> GSAMGQNPWATTTAFADFMKRFNIPQVHGSGIFVDLGRDTEGYREVGGKCPVFGKAIQMHQPAEYSNNFLDDAPTSNDASKKPLPGGFNNPQVYTSGQKFSPIDDSLLQERLGTAGPKTAIGRCALYAYSTIAVNPSTNYTSTYKYPFVYDAVSRKCYVLSVSAQLLKGEKYCSVNGTPSGLTWACFEPVKEKSSARALVYGSAFVAEGNPDAWQSACPNDAVKDALFGKWEDGQCVPFDTKTSVQSDQATNKEECWKRVFANPLVASDAPTTYPEAAQKNWNDFWPVHEQSSPKSGGFGANWANFYLEKESGETICAIFDQVPDCFAPITGAVAYTALGSSTEVNLPQCDSASFIPIEGPCNNCVQVVTECVGNQFDQTSKACCTEPEAAALVPR;> GSASDIAQFLTDSGMKAIEDCSWNPIMQQMACVVVAGSGS

AMA1, a type I transmembrane protein, is conserved across all Apicomplexans and its knockdown has been shown to markedly reduce invasion. Recently, Toxoplasma sporozoites were subjected to detailed transcriptomic and proteomic analyses. It was found that, in addition to the well-characterized “generic” AMA1 and RON2, sporozoites also express two paralogues dubbed sporoAMA1 and sporoRON2, respectively, that are not expressed at detectable levels in tachyzoites or bradyzoites. To better understand the mutually exclusive nature of the interaction between the sporozoite and generic AMA1/RON2 pairings, we set out to solve the crystal structure of apo sporoAMA1 and of sporoAMA1 bound to a portion of sporoRON2-D3 (sD3). The results presented here demonstrate that invasion of Toxoplasma sporozoites depends on the interaction of two previously uncharacterized proteins, sporoRON2 and sporoAMA1.

The co-structure of sporoAMA1 with sporoRON2-D3 reveals significant complementarity, with a buried surface area of 3274 Å2, 23 intermolecular hydrogen bonds, and a complexation significance score of 1.00 indicating physiological relevance. SporoRON2-D3 is integrated into the apical groove of sporoAMA1 through an N-terminal α-helix seated in the area exposed by displacement of the domain II loop and connecting coil ordered through the center of the groove to the disulfide-bound beta hairpin loop at the opposite end of the apical surface. Nearly three quarters of the hydrogen bonds formed between sporoAMA1 and sporoRON2-D3 are found within the cysteine loop region, and only the strictly backbone interactions are observed at the generic AMA1-generic RON2sp interface, which contains approximately half the number of hydrogen bonds observed for generic AMA1 and the generic RON2 cysteine loop. Firstly, sporoRON2 Met1009 buries into a deep cleft in the side of sporoAMA1, while the corresponding residue in generic RON2 is Gly1307 and there is no cleft in this region of generic AMA1 due to the presence of Met233. Secondly, beta-hairpin loop 3 is four residues shorter in sporoAMA1 than generic AMA1, which together with the introduction of a glutamic acid residue in this loop (sporoAMA1 Glu132), presents an enlarged pocket with sufficient shape and charge complementarity to accommodate an extended lysine residue of sporoRON2 (sporoRON2 Lys1010). Finally, the flattened surface caused by the presence of groove-central Ser252 in sporoAMA1 readily accommodates a bowed out conformation of sporoRON2-D3 consisting of Ile1012 and Glu1013, whereas the corresponding central residue in generic AMA1, Tyr230, limits the accessible area in this region and can only accommodate a valine (Val1311) flipped down towards the base of the groove and held in position by Pro1310. The C-terminus of sporoRON2-D3, for example, does not extend the length of the groove as observed in the generic AMA1-RON2sp co-structure, but rather exits the groove shortly after the disulfide of the beta hairpin loop.> IRPRKKGMRLDRRRSKKQYK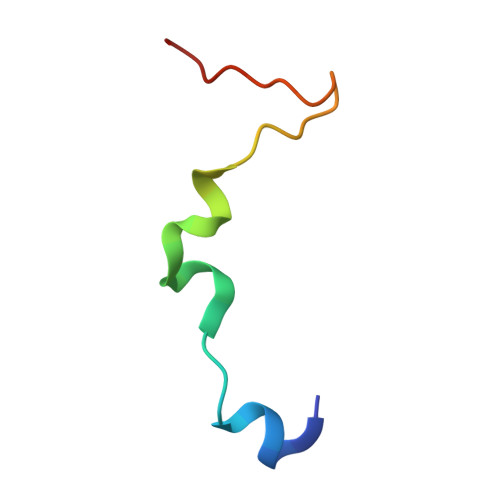HGRHVGGWNYRWLGS>[3x]HHHHHHSSGMASINLPFSLSGSKRIPTSEELADGYQCGPLDVELDNWLMWWLTGQVDGVIEGA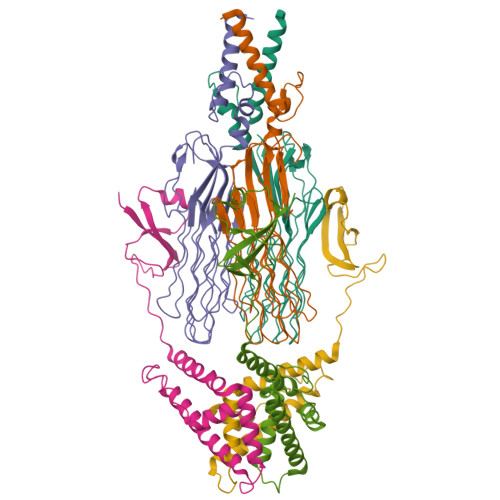GLTTDDTDLARLYKAIQSMTSGNLRTVVLTAASGNLPIPSDVSVLNWVRAVGGGGAGGNSNTGNSKASGGGGGAGFDRFNVAVTPGSNVPYTVGAAGAVNGLGAGYNGGAGGSTAILGTTAGGGAGGLGVNNNATAVQVNGGTTSGTTPEISYPGGLGTEGIVGTGGGSVLSQPTQRAFTNAGNNNPANSWGGGGPGGSDFGGAWQPGGVGKQGIIIVQYFSRFAP;>MTDKHYARVVDGLVVETKTLPADFNLDDLFGPDHGWVEAPLEVEQGWRKVGAKFAPAPPPERDPASILAGLKAEASRHIFATISATAQSNLLLAVGLASAKAPSARTPEERDLLNVADEGRAWIDAVRARVHALAEHDGVTPKGEDRWPAPSEAVLEMAAKF[3x]> GGFQVVTFEWAHVQDPYVIALWILVASLAKIGFHLSHKVTSVVPESALLIVLGLVLGGIVWAADHIASFTLTPTVFFFYLLPPIVLDAGYFMPNRLFFGNLGTILLYAVVGTVWNAATTGLSLYGVFLSGLMGDLQIGLLDFLLFGSLMAAVDPVAVLAVFEEVHVNEVLFIIVFGESLLNDAVTVVLYNVFESFVALGGDNVTGVDCVKGIVSFFVVSLGGTLVGVVFAFLLSLVTRFTKHVRIIEPGFVFIISYLSYLTSEMLSLSAILAITFCGICCQKYVKANISEQSATTVRYTMKMLASSAETIIFMFLGISAVNPFIWTWNTAFVLLTLVFISVYRAIGVVLQTWLLNRYRMVQLEPIDQVVLSYGGLRGAVAFALVVLLDGDKVKEKNLFVSTTIIVVFFTVIFQGLTIKPLVQWLKVKRSEHREPR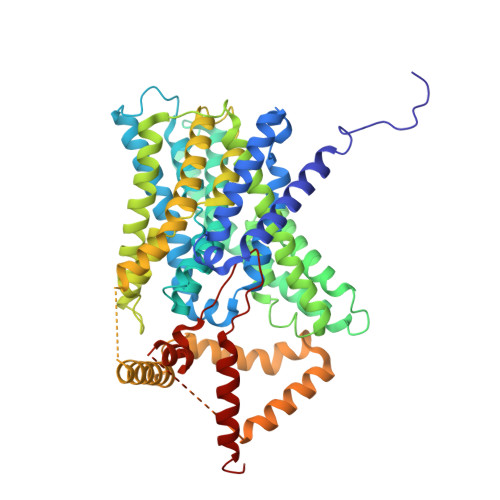LNEKLHGRAFDHILSAIEDISGQIGHNYLRDKWSHFDRKFLSRVLMRRSAQKSRDRILNVFHELNLKDAISYVAEGERRGSLAFIRSPSTDNVVNVDFTPRSSTVEASVSYLLRENVSAVCLDMQSLEQRRRSIRDAEDMVTHHTLQQYLYKPRQEYKHLYSRHELTPTEDEKQDREIFHRTMRKRLESFK> MGSDKIHHHHHHMKVFVIGAGLMGRGIAIAIASKHEVVLQDVSEKALEAAREQIPEELLSKIEFTTTLEKVKDCDIVMEAVFEDLNTKVEVLREVERLTNAPLCSNTSVISVDDIAERLDSPSRFLGVHWMNPPHVMPLVEIVISRFTDS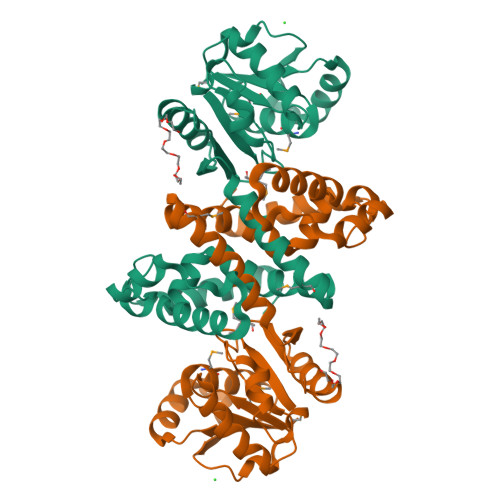KTVAFVEGFLRELGKEVVVCKGQSLVNRFNAAVLSEASRMIEEGVRAEDVDRVWKHHLGLLYTLFGPLGNLDYIGLDVAYYASLYLYKRFGDEKFKPPEWLQEKIKKGEVGVKAGKGIYEYGPKAYEERVERLKKLLRFLGLE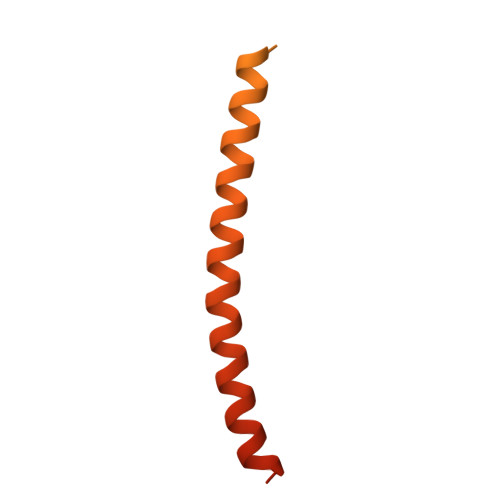> MDEASHLPNGSLKNMEFTPVGFIKSKRNTTQTQVVSPTKVPNANNGDENEGPVKKRQRRSIDDTIDSTRLFSEASQFDDSFPEIKANIPPSPRSGNVDKSRKRNLIDDLKKDVPMSQPLKEQEVREHQMKKERFDRALESKLLGKRHITYANSDISNKELYINEIKSLKHEIKELRKEKNDTLNNYDTLEEETDDLKNRLQALEKELDAKNKIVNSRKVD> MPEGPELHLASQFVNEACRALVFGGCVEKSSVSRNPEVPFESSAYRISASARGKELRLILSPLPGAQPQQEPLALVFRFGMSGSFQLVPREELPRHAHLRFYTAPPGPRLALCFVDIRRFGRWDLGGKWQPGRGPCVLQEYQQFRESVLRNLADKAFDRPICEALLDQRFFNGIGNYLRAEILYRLKIPPFEKARSVLEALQQHRPSPELTLSQKIRTKLQNPDLLELCHSVPKEVVQLGGRGYGSESGEEDFAAFRAWLRCYGMPGMSSLQDRHGRTIWFQGDPGPLAPKGRKSRKKKSKATQLSPEDRVEDALPP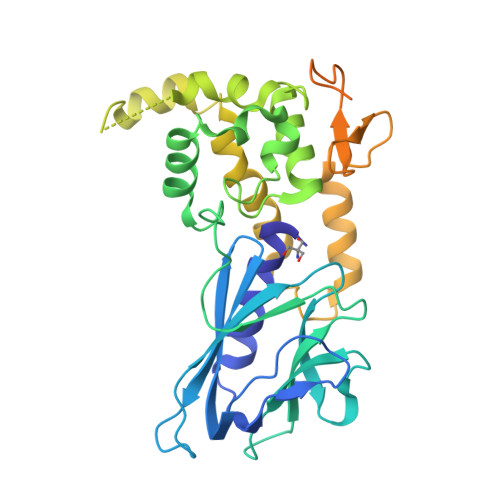SKAPSRTRRAKRDLPKRKGRQAASGHCRPRKVKADIPSLEPEGTSAS> MTHLERSRHQQHPFHMVMPSPWPIVVSFALLSLALSTALTMHGYIGNMNMVYLALFVLLTSSILWFRDIVAEATYLGDHTMAVRKGINLGFLMFVLSEVLIFAGLFWAYFHSAMSPDVTLGACWPPVGIEAVQPTELPLLNTIILLSSGATVTYSHHALIAGNRNKALSGLLITFWLIVIFVTCQYIEYTNAAFTISDGVYGSVFYAGTGLHFLHMVMLAAMLGVNYWRMRNYHLTAGHHVGYE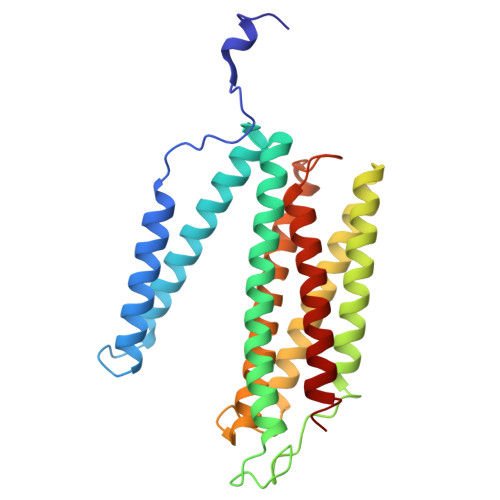TTIIYTHVLDVIWLFLYVVFYWWGV N~2~-[(4-fluoro-3-methoxyphenyl)sulfonyl]-N-hydroxy-N~2~-(2-methylpropyl)-D-valinamide 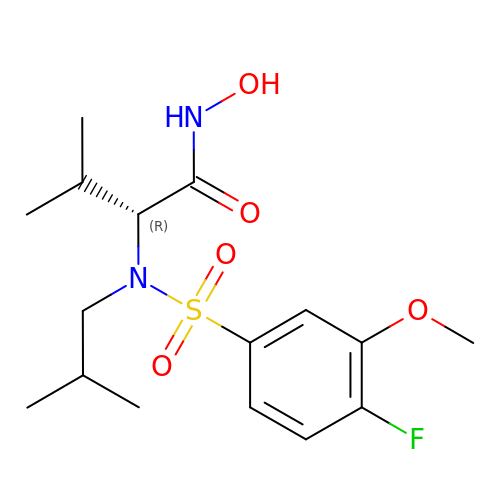| C16 H25 F N2 O5 S | GINWIYLMIMGVMO-OAHLLOKOSA-N> VPDPRGIIINLDEGELCLNSAQCKSNCCQHDTILSLLRCALKARENSECSAFTLYGVYYKCPCERGLTCEGDKSLVGSITNTNFGICHNVGRSDS;> KEVCYERLGCFSDDSPWSGITERPLHILPWSPKDVNTRFLLYTNENPNNFQEVAADSSSISGSNFKTNRKTRFIIHGFIDKGEENWLANVCKNLFKVESVNCICVDWKGGSRTGYTQASQNIRIVGAEVAYFVEFLQSAFGYSPSNVHVIGHSLGAHAAGEAGRRTNGTIGRITGLDPAEPCFQGTPELVRLDPSDAKFVDVIHTDGAPIVPNLGFGMSQVVGHLDFFPNGGVEMPGCKKNILSQIVDIDGIWEGTRDFAACNHLRSYKYYTDSIVNPDGFAGFPCASYNVFTANKCFPCPS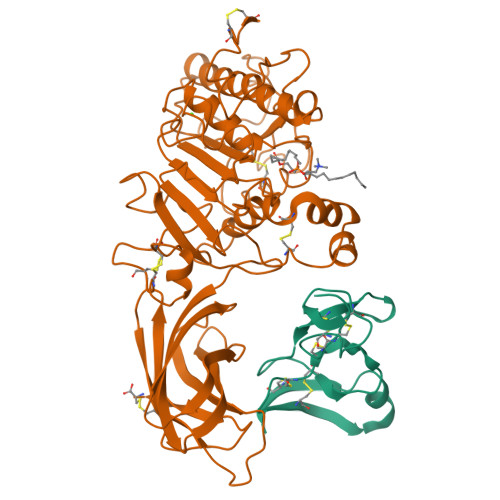GGCPQMGHYADRYPGKTNDVGQKFYLDTGDASNFARWRYKVSVTLSGKKVTGHILVSLFGNKGNSKQYEIFKGTLKPDSTHSNEFDSDVDVGDLQMVKFIWYNNVINPTLPRVGASKIIVETNVGKQFNFCSPETVREEVLLTLTPC>SA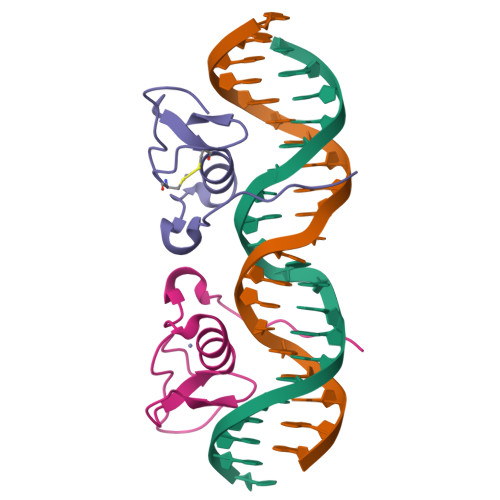ARRAGTSCANCQTTTTTLWRRNANGDPVCNACGLYYKLHNINRPLTMKKEGIQTRNRKMSS[2x]> TCGGC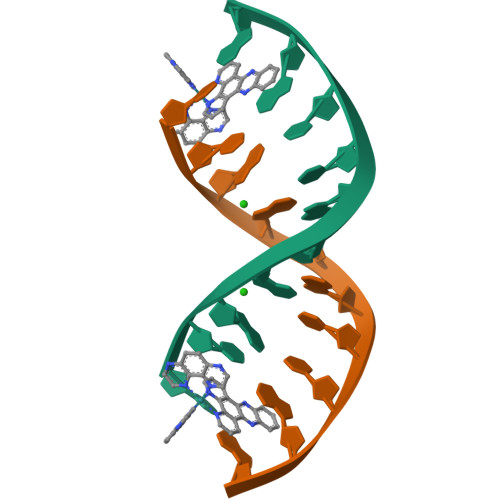ICCGA> DTVGRPLPHLAAAMQASGEAVYCDDIPRYENELFLRLVTSTRAHAKIKSIDVSEAQKVPGFVCFLSADDIPGSNETGLFNDETVFAKDTVTCVGHIIGAVVADTPEHAERAAHVVKVTYEDLPAIITIEDAIKNNSFYGSELKIEKGDLKKGFSEADNVVSGELYIGGQDHFYLETHCTIAIPKGEEGEMELFVSTQNAMKTQSFVAKMLGVPVNRILVRVKRMGGGFGGKETRSTLVSVAVALAAYKTGHPVRCMLDRNEDMLITGGRHPFLARYKVGFMKTGTIVALEVDHYSNAGNSRDLSHSI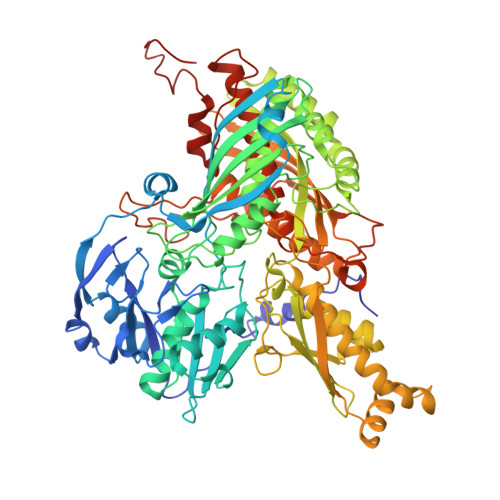MERALFHMDNCYKIPNIRGTGRLCKTNLSSNTAFRGFGGPQALFIAENWMSEVAVTCGLPAEEVRWKNMYKEGDLTHFNQRLEGFSVPRCWDECLKSSQYYARKSEVDKFNKENCWKKRGLCIIPTKFGISFTVPFLNQAGALIHVYTDGSVLVSHGGTEMGQGLHTKMVQVASKALKIPISKIYISETSTNTVPNSSPTAASVSTDIYGQAVYEACQTILKRLEPFKKKNPDGSWEDWVMAAYQDRVSLSTTGFYRTPNLGYSFETNSGNAFHYFTYGVACSEVEIDCLTGDHKNLRTDIVMDVGSSLNPAIDIGQVEGAFVQGLGLFTLEELHYSPEGSLHTRGPSTYKIPAFGSIPTEFRVSLLRDCPNKKAIYASKAVGEPPLFLGASVFFAIKDAIRAARAQHTNNNTKELFRLDSPATPEKIRNACVDKFTTLCVTGAPGNC> MFEKGYVDENYIRVPKDRLFSFIVRVLTKLGVPEEDAKIVADNLVMADLRGVESHGVQRLKRYVDGIISGGVNLHPKIRVIREGPSYALIDGDEGLGQVVGYRSMKLAIKKAKDTGIGIVIARNSNHYGIAGYYALMAAEEGMIGISMTNSRPLVAPTGGIERILGTNPIALAAPTKDKPFLLDMATSVVPIGKLEVYRRKGKDIPEGWAINREGNITTKVEEVFNGGALLPLGGFGELLGGHKGYGLSLMVDILSGILSGGTWSKYVKNTSEKGSNVCHFFMVIDIEHFIPLEEFKEKISQMIEEIKSSRKHPEFERIWIHGE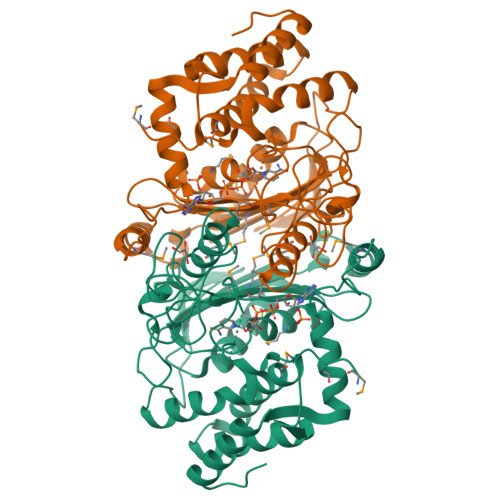KGFLTMETRLKLGIPIYRKVLEELNEIAKRVGVEGL> NPRAQVFEYFKLKVPATRGAVLKAHINHLGNVAAMVSFILVHHLSWDPATQGVLWAPATMFYARLYQLGLDAVALSPDALFVARMHLLAAIILWGFGHVKSPAEEKFLEKVTMGKALVAQFHFFALIATLWGLHMAFYGILGPSGKLEPTGLSFDM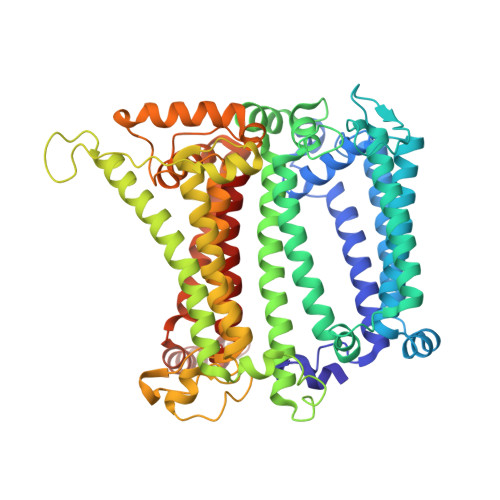FGPITPATMAGNHVAFGAVFFLGGIFHYFAGFNTKRFAFFEKDWEAVLSVSCQILAFHFATVVFAMIIWQHPQLGFGFMREYAVSQYAGPELKMIAQSNPGLLVKQAILGHLVMGIMFWIGGVFHGAHFMLRVLNDPKLAEEMKDFKFIKRCYDHEFQKKFLALIMFGAFLPIFVSYGIATHNTIADIHAASKTGLFAHMTYINIGTPLHDAIFGSKGSISEFVAAHAIAGGLHFTMVPMWRMVFFSKVSPWTTKVGMKAKRDGEFPCLGPAYGGTCSISLVDQFYLAIFFSLQVIAPAWFYIDGCWMGSFVAVAAPYNDIYQAALATFNSHNPLHQLSPLTNMGYFSYIIQQTTAMFSRYDGHMIQALLGAHFIWAFTFSMLFQYRGSRDEGAMVLKWAHQQVGVGFAGKMYNRALSLKEGKAIGCFLFFKMTIVCMWALAMV> MKKTLPTKKSNLWFLMACLIITFHKVEAQVPDPNQGLRAEWMRGALGMLWLPERTFNGNIEGIRIDDFLTQIKDIRTVDYVQLPLTSPNIFS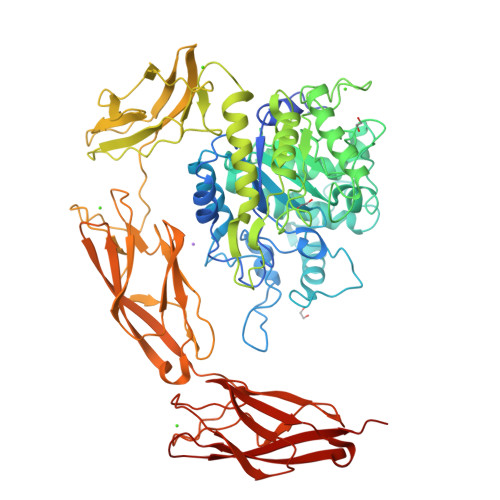PTHVAPHPIIESLWQGDTDANGDPINLVAPRESVDDPLLSWLKALRAAGLRTEIYVNSYNLLARIPEDTQADYPDVSARWMEWCDTNTEAQAFINSQTYHEGNGRRKYMFCYAEFILKEYAQRYGDLIDAWCFDSADNVMEDECGDDPASEDVNDQRIYQAFADACHAGNPNAAIAFNNSVGDREGNPFTSATLFDDYTFGHPFGGAGNMVVPEALYTYNHDLVVFMQTNNGYAFRDDTRTWNDNVVAHFFPKQSTTSWNAGNTPCLTDEQFVEWTSTGIVNGGGITWGTPLVRTNLENAPVLTLQPYALNQFELTDTYLKEFQSPGKPNWSRQYTILPAIYPGQPYSHNLVEGVDFWDPEGVGITGLTASGTLPAWLTISQTATGTWTLSGTPPVSEASNYTFELMAQDSDGVTNREVKLEVISHPAGFTNPGDGTPVWFSNPMVLAKATALKDYGSLLKLGVDFYDFEGDVLTITKTSGPDWLVLTQNSDDTWRLSGMPTAADAGENSFTFNVSDGILSSDTEIKITVDHVAGFTNLGNGAPVWSSPILNLTDGKGSFAYNYTLQLGTDYYDFEGDALTITKTSGPDWLTIQQTDANSWKLSGTPINSDAGENSFTFNLSDDTNSTTAEILINVIATIIS>GPGMKDCSNGCSAECTGEGGSKEVVGTFKAKDLIVTPATILKEKPDPNNLVFGTVFTDHMLTVEWSSEFGWEKPHIKPLQNLSLHPGSSALHYAVELFEGLKAFRGVDNKIRLFQPNLNMDRMYRSAVRATLPVFDKEELLECIQQLVKLDQEWVPYSTSASLYIRPTFIGTEPSLGVKKPTKALLFVLLSPVGPYFSSGTFNPVSLWANPKYVRAWKGGTGDCKMGGNYGSSLFAQCEAVDNGCQQVLWLYGEDHQITEVGTMNLFLYWI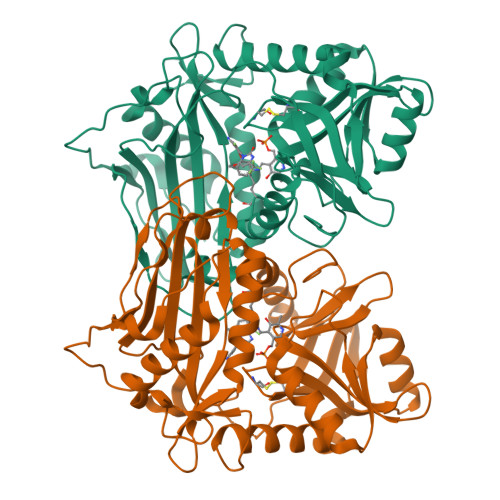NEDGEEELATPPLDGIILPGVTRRCILDLAHQWGEFKVSERYLTMDDLTTALEGNRVREMFGSGTACVVCPVSDILYKGETIHIPTMENGPKLASRILSKLTDIQYGREERDWTIVLS[4x]> ADVPAGVQLADKQTLVRNNGSEVQSLDPHKIEGVPESNVSRDLFEGLLISDVEGHPSPGVAEKWENKDFKVWTFHLRENAKWSDGTPVTAHDFVYSWQRLADPNTAS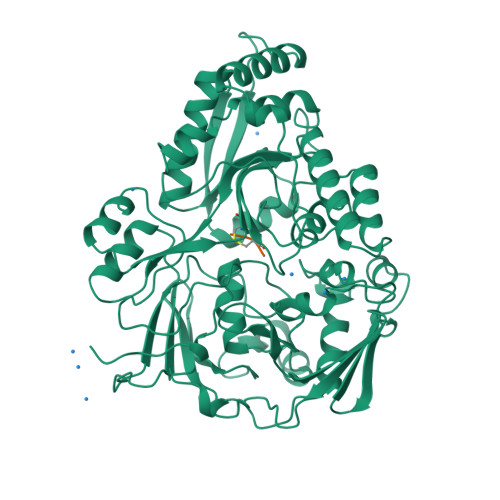PYASYLQYGHIANIDDIIAGKKPATDLGVKALDDHTFEVTLSEPVPYFYKLLVHPSVSPVPKSAVEKFGDKWTQPANIVTNGAYKLKNWVVNERIVLERNPQYWDNAKTVINQVTYLPISSEVTDVNRYRSGEIDMTYNNMPIELFQKLKKEIPNEVRVDPYLCTYYYEINNQKAPFNDVRVRTALKLALDRDIIVNKVKNQGDLPAYSYTPPYTDGAKLVEPEWFKWSQQKRNEEAKKLLAEAGFTADKPLTFDLLYNTSDLHKKLAIAVASIWKKNLGVNVNLENQEWKTFLDTRHQGTFDVARAGWCADYNEPTSFLNTMLSDSSNNTAHYKSPAFDKLIADTLKVADDTQRSELYAKAEQQLDKDSAIVPVYYYVNARLVKPWVGGYTGKDPLDNIYVKNLYIIKH;> KEK> MAQQSTKNETALLVAKSAKSALQDFNHDYSKSWTFGDKWDNSNTMFETFVNKYLFPKINETLLIDIALGNRFNWLAKEQDFIGQYSEEYVIMDTVPINMDLSKNEELMLKRNYPRMATKLYGNGIVKK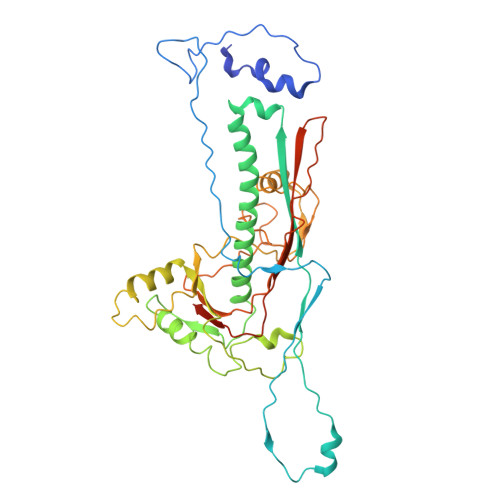QKFTLNNNDTRFNFQTLADATNYALGVYKKKISDINVLEEKEMRAMLVDYSLNQLSETNVRKATSKEDLASKVFEAILNLQNNSAKYNEVHRASGGAIGQYTTVSKLKDIVILTTDSLKSYLLDTKIANTFQIAGIDFTDHVISFDDLGGVFKVTKEFKLQNQDSIDFLRAYGDYQSQLGDTIPVGAVFTYDVSKLKEFTGNVEEIKPKSDLYAFILDINSIKYKRYTKGMLKPPFHNPEFDEVTHWIHYYSFKAISPFFNKILITDQDVNPKPEEELQE> VSDALDEGLVQRIDARGTIEWSETCYRYTGAHRDALSGEGARRFGGRWNPPLLFPAIYLADSAQACMVEVER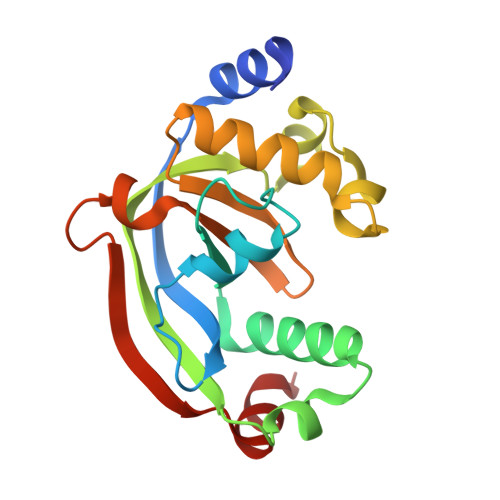AAQAASTTAEKMLEAAYRLHTIDVTDLAVLDLTTPQAREAVGLENDDIYGDDWSGCQAVGHAAWFLHMQGVLVPAAGGVGLVVTAYEQRTRPGQLQLRQSVDLTPALYQELRAT(1~{R},2~{R})-~{N}-(1~{H}-pyrazol-4-yl)-2-pyridin-3-yl-cyclopropane-1-carboxamide 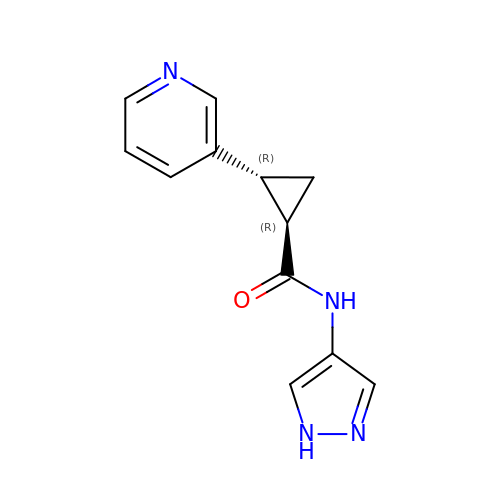| C12 H12 N4 O | ONPYJJLGIGTZEH-WDEREUQCSA-N> GELIQKYIDEILAEAEAGKKLLLIGAGPAAAKAAIEEAMKRLAETLEELLGVEVKVEIVDDGEYEKAAKII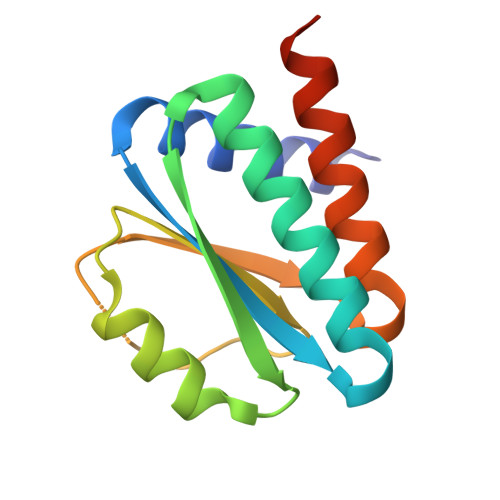KEADADVVVFISTKELKKIDTKAKLINILAADADKVAVLDALIAAARARALEHHHHHH> MRRFAAGCLALALLVLPFVLTGARAAEDESEKEIERYRQMIEDPMANPGFLNVDRGEVLWSEPRGTRNVSLETCD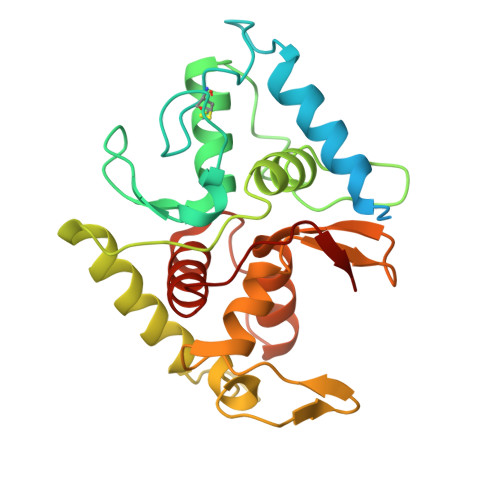LGEGPGKLEGAYAHLPRYFADTGKVMDLEQRLLWCMETIQGRDTKPLVAKPFSGPGRTSDMEDLVAFIANKSDGVKIKVALATPQEKEMYAIGEALFFRRSSINDFSCSTCHGAAGKRIRLQALPQLDVPGKDAQLTMATWPTYRVSQSALRTMQHRMWDMYRQMRMPAPDYASEAVTALTLYLTKQAEGGELKVPSIKR>[2x]MSKPPKELIARTGRVQSWIDDPTSRLPVSCTVFVVEDTMEGENGIEASWRFVSHALRYGAGVAVHLSKLRPKGAENGKGLVASGPVSFAKIYSTLNEILRRGGVYKNGAVVCHLDLSHPDVLEFITASRSELPWVKRCVNINDHWWKEATPTVKNALLEGIKRGDIWLNKTKVDRNGNRIRGNVCLEVYLPSRGTCLLQHVNLGGCELDEIRGAFAQGMSELCELHGKTNVGESGEYLPSETDRQVGLGMLGLANLLRTQGVTYNDFGRALEALNSGRPYPSTPGYVIAQELKAGIQAAAEIAKANKMERAFAIAPTASCSYRYTDLDGYTTCPEIAPPIARQVDRDSGTFGVQSFDYGPVEIASEVGWESYKRVVDGIIRLLDSTGLLHGYSFNSWSDVVTYDEQFIEDWLASPQTSLYYSLQVMGDVQDKSDAYAALDDGDVTAYLESLLNDPVGASPPLAPDCNCGE

RNRs are used by all free-living organisms and many viruses for the conversion of ribonucleotides to 2ʹ-deoxyribonucleotides in the de novo biosynthesis of DNA precursors. RNRs are especially fascinating from an evolutionary perspective as they exhibit high diversity in primary sequence and cofactor requirement, yet they share a common fold and radical-based catalytic mechanism for nucleotide reduction. Despite being a diverse enzyme family, the core structure of the catalytic subunit (known as α) is a conserved 10-stranded α/β barrel with the thiyl radical on the so-called ‘finger loop’ which connects the two halves of the barrel (Uhlin and Eklund, 1996). Our comprehensive phylogeny shows the parallel development of three major clades, corresponding to the three known classes, with a small, phylogenetically distinct clade, which we denote as class Ø (for convenience, pronounced ‘oh’), placed as an ancestral clade to the class I and II RNRs.

To examine the structural features of the class Ø RNR, we used a combination of AlphaFold2, SAXS, and cryo-EM to characterize the Synechococcus phage S-CBP4 α subunit. Addition of substrate (guanosine diphosphate [GDP]) does not shift this equilibrium, but the presence of the corresponding specificity effector (thymidine triphosphate [TTP]), strongly favors dimerization. Using solution conditions that saturate nucleotide binding (200 μM TTP, 200 μM GDP), we obtained a cryo-EM map of the S-CBP4 α2 dimer to 3.46 Å resolution (Fourier shell correlation [FSC] = 0.143). An atomic model (residues 22–426 out of 470) was refined against the cryo-EM map using an AlphaFold2 prediction as the starting model. Overall, the S-CBP4 α subunit displays the most minimal RNR architecture discovered to-date with few insertions about the catalytic barrel. The minimal set of insertions includes traits shared by class I and II RNRs, such as loop 1, where we find cryo-EM density for bound TTP. Additionally, the S-CBP4 α subunit contains a long β-hairpin following the βH strand of the catalytic barrel that in class II RNRs is thought to be important for cofactor binding and in class I RNRs is thought to be important for interactions with the β subunit. Although we do not observe density for the C-terminus past the βJ strand of the catalytic barrel, two consecutive tyrosine residues (Y420 and Y421) on βJ are well resolved and stacked adjacent to the catalytic cysteine (C185) at the tip of finger loop. Finally, we observe a disulfide between active-site cysteines (C30 and C196) that in class I and II RNRs serve as reducing equivalents during nucleotide reduction. Consistent with an oxidized active site, cryo-EM density for the substrate is not observed.> MAETFKIRKLEISDKRKGFIELLGQLTVTGSVTDEEFDRRFEEIRSYGDDHVICVIEEETSGKIAATGSVMIEKKFLRNCG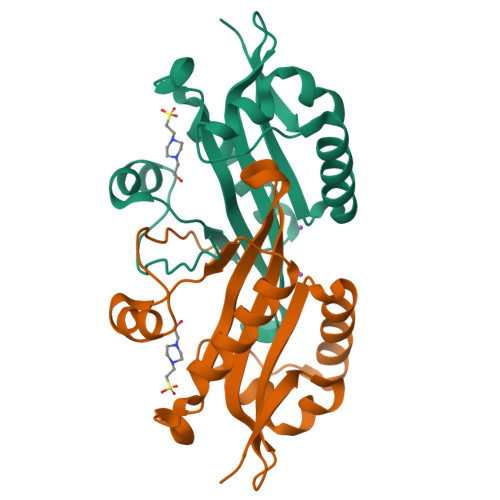KAGHIEDVVVDSRFRGKQLGKKVVEFLMDHCKSMGCYKVILDCSVENKVFYEKCGMSNKSIQMSKYFD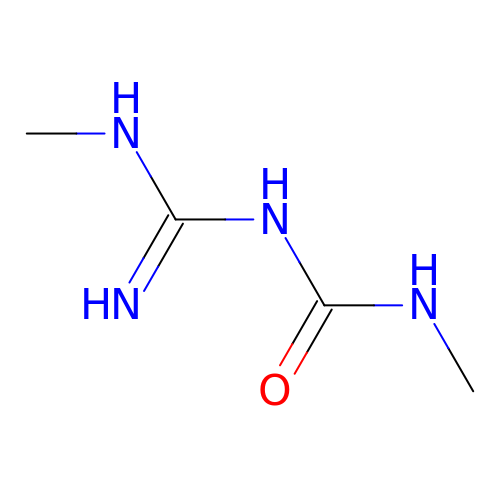1-methyl-3-(N-methylcarbamimidoyl)urea | C4 H10 N4 O | KGCIDHJBLPVUNN-UHFFFAOYSA-N>[2x]DRHHH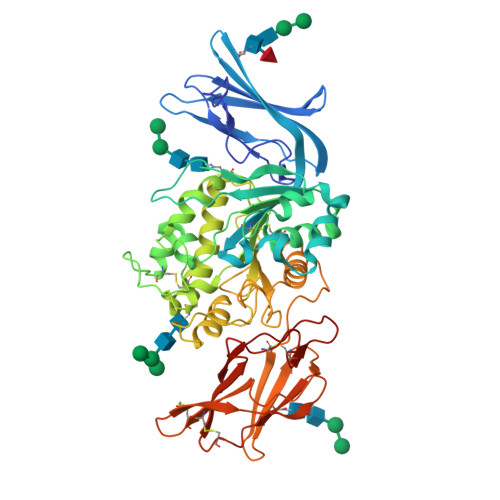HHHKLIGFRFASYIDNYMVLQKEPAGAVIWGFGIPGATVTVTLCQGQQAIMKKVTSVKAHTNTWMVVLDPMKPGGPYEVMAQQSLWSRNFTVQVHDVLFGDVWLCSGQSNMQMTVLQIFNAVRELSDTAAYQSVRLLSVSLTEAEEELQDLNAVDLQWSKPTKENLGNGDFTYMSAVCWLFGRYLYDTLQYPIGLISSCWGGTPIEAWSSERSLKACGVPTKGSLLSDSVSGPSQNSILWNAMIHPLQNMTLKGVLWYQGESNVNYNKDLYNCTFPALIEDWRQTFHSGSQGQTERVFPFGFVQLSSYLSTADDPPVGVPQIRWHQTADLGFVPNRRMPNTFMAVALDLCDRTSPFGSIHPRDKQTVAYRLHLGARAVAYGEKNLTFQGPLPEKIELLSTDGLLNLTYHQSIQVLRQDLQIFEISCCSDRQCKWLPAPMNTFTSQTLTLSIRSCRGTVAAVRYAWTPWPCEYKQCPLYHPSSALPAPPFLAFITDQASRH>MVKLRDLDIIVTAPPAPGWGGRYWILVKLTTDDGITGWGECYAASVGPEAMRAVIEDVFARHMEGENPENIELMFRRVYSSGFTQRPDLTAIGAFSGLEIACWDILGKARGRPVWALLGGKMNPRIRAYTYLYPLPHHPITPFWTSADMAAESAADCVARGYTAVKFDPAGPYTLRGGHMPAMTDISLSVEFCRKIRAAVGDKADLLFGTHGQFTTAGAIRLGQAIEPYSPLWYEEPVPPDNVGAMAQVARAVRIPVATGERLTTKAEFAPVLREGAAAILQPALGRAGGIWEMKKVAAMAEVYNAQMAPHLYAGPVEWAANVHFAASIPNILMCESIETPFHDALIKGSIRVEGGYITPPEAPGLGIEVDEALARANP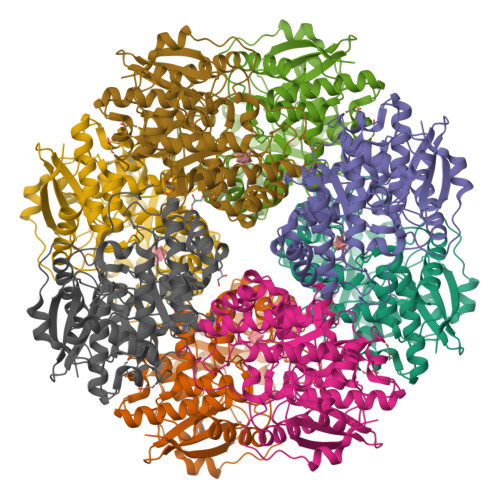YHGTGLHLEMQEASCDYTNGNSFAGGAPHEEGAENLYFQSHHHHHHWSHPQFEK[8x]8,9-DICHLORO-2,3,4,5-TETRAHYDRO-1H-BENZO[C]AZEPINE | 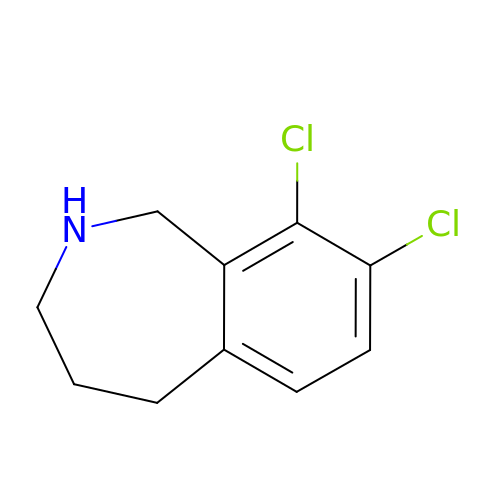C10 H11 Cl2 N | IADAQXMUWITWNG-UHFFFAOYSA-N>GCAGXCUUAAGUCU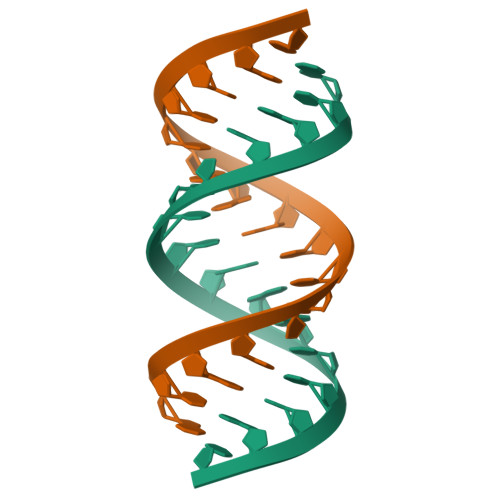GC[3x]>[4x]GSHMMEFKTDIEIAQEANPQDIRDIAKKINLSEDDIELYGKYKAKIDYNVLNRTKSRAGKLILTTAINPTPAGEGKTTTSIGVADALAKLGKNVIAALREPSMGPVFGIKGGAAGGGYAQVVPMEDINLHFTGDMHAIGAANNLLAAMLDNHVYQTNSLNINPKRITWRRCVDMNDRQLRNVVDGLGKKVDGVTREDGFDITVASEVMAAFCLSNNISELKENLGNIVVAYNYSGKPVTARDLNAHGAMAAILKDALKPNLVQTLEGTPAILHGGPFANIAHGCNSIIATKMGMHMADYVVTEAGFGADLGAEKFLDIKCRKAGIRPDAVIIVATVRALKYNGGVAKDQLNNENLEALEKGLPNLLKHIENITQVYKIPAVVAINRFPLDTDAELALVRSKCEELGVKVALSEVWANGGEG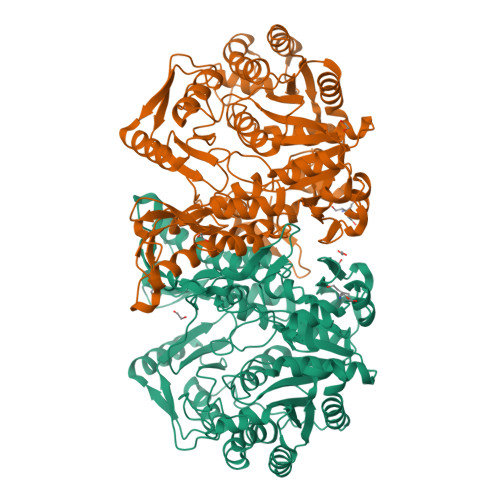GIEVANEVLKLIEEGENNFEYCYEEDMTIKEKLNAIATKIYGADGVNYTKEANKQIAELEELGFGNLPVCVAKTQYSLSDDQTKLGRPTGFTIEVRQANISAGAGFVVVMTGEIMKMPGLPKLPAAERIDVDENGKISGLF> RPQGATVSLWETVQKWREYRRQCQRSLTEDPPPATDLFCNRTFDEYACWPDGEPGSFVNVSCPWYLPWASSVPQGHVYRFCTAEGLWLQKDNSSLPWRDLSE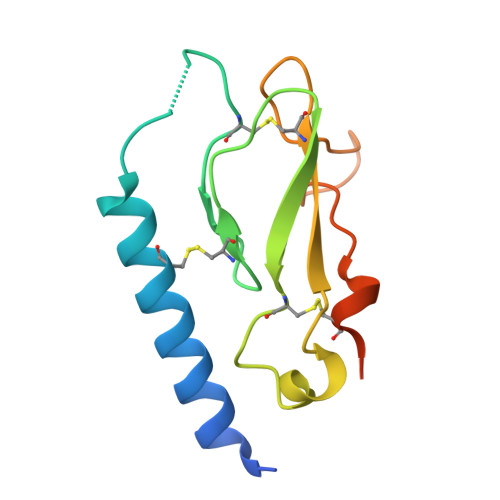CEESKRGERSSPEE> GSMEPAMEPETLEARINRATNPLNKELDWASINGFCEQLNEDFEGPPLATRLLAHKIQSPQEWEAIQAL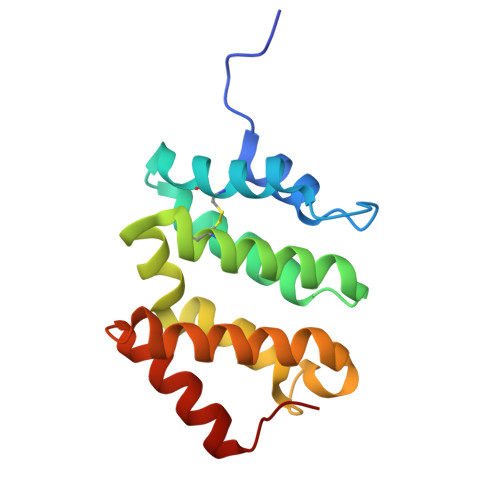TVLETCMKSCGKRFHDEVGKFRFLNELIKVVSPKYLGSRTSEKVKNKILELLYSWTVGLPEEVKIAEAYQMLKKQGIVKS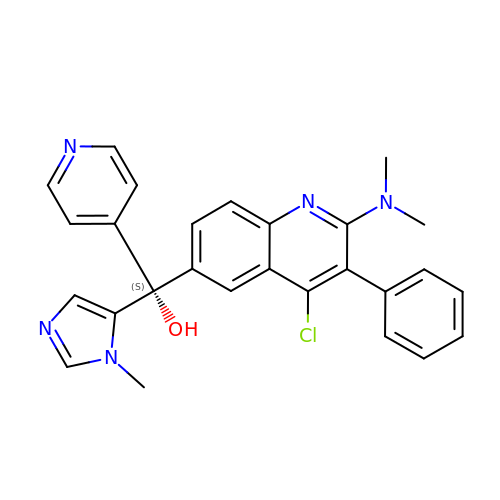(S)-[4-chloro-2-(dimethylamino)-3-phenylquinolin-6-yl](1-methyl-1H-imidazol-5-yl)(pyridin-4-yl)methanol | C27 H24 Cl N5 O | SEJAMGYPDDPTHR-HHHXNRCGSA-N>[2x]MMKPEDVIKEQCARAKVVAELWHGFTGGAPKAALENLVVEFNKAQQGRCVRPVPQGGYRDLSTKIKAAFAAGKVPTMAQAFENNIALYLEAKALLPIESLGVKLQGVNLTFLNAVRFGGV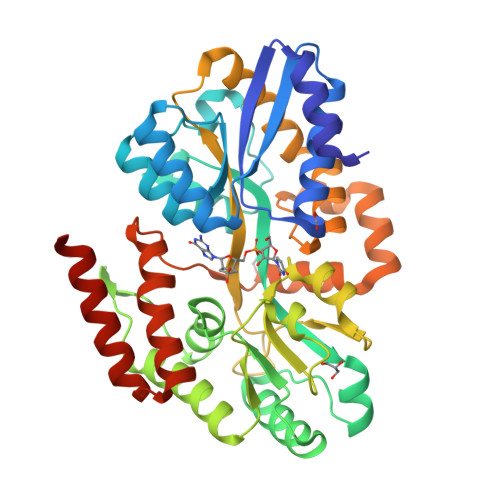VYGVPFNKSIQVLYYNKDLLKKHGVPVPATLEEFVAAAKKLSRAEGGPVYWFQPDASTFAYFFFNLGGSYLKDGKLVLNSKEAVEALTLLQNGVKEGWAKPITSGAINQNLGSGPYAFSVDTSAGYTYYLRAAKFDLGVATLPGRTKGQPGYGLVQGTNLVVFRQASKEEQAVAKDFLEFVLSPRAQAVFATATGYVPVTEGALKDPVYQAYAAENPDYATIVRQSRYAKFEPALAEWEQIRFDILGQAIKEAILNKADPKAALDRAQKLAEDLLSSRTRHHHHHH>NKSDAAAKQIKKLEEDFDGRIGVFAIDTGSGNTFGYRSDER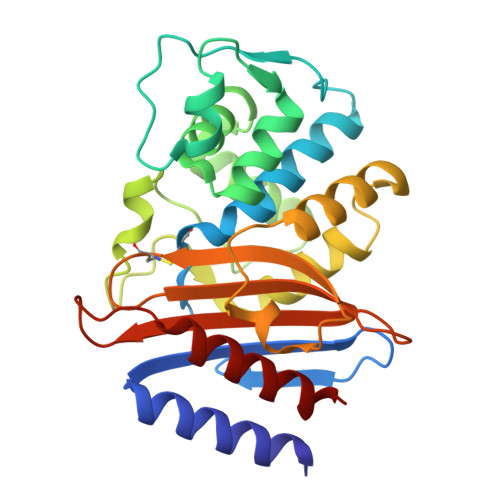FPLCSSFKGFLAAAVLERVQQKKLDINQKVKYESRDLEYHSPITTKYKGSGMTLGDMASAALQYSDNGATNIIMERFLGGPEGMTKFMRSIGDNEFRLDRWELELNTAIPGDKRDTSTPKAVANSLNKLALGNVLNAKVKAIYQNWLKGNTTGDARIRASVPADWVVGDKTGSCGAYGTANDYAVIWPKNRAPLIVSIYTTRKSKDDKHSDKTIAEASRIAIQAID[2x]> MGHHHHHHGENLYFQGSMHEHFDSIYLEFVDESYKPGKDEVIAVFRVTPAQGISIKDAAGRIAAESSVGTWTTLSVKPSWFEKLKAKAYRFHDLGDGSWLVWVAYPVELFEEGSIPNFASSILGNIFGMKAIAGLRVEDVYFPPSYLETFPGPNKGIQGVREILGIKDRPILATVPKPKLGYTPEEYGRVAYEILIGGIDLVKDDENFASQPFCRFEARLKEVMKAIDRAEKETGERKGYLANVTAPIREMEKRIKLVADYGNKFIMIDFLTAGWAALQHARELAEEYDLAIHGHRAFHAAFTRNPKHGVSMFLVAKLARMAGVDHVHVGTPGVGKMDAKTREVLEHTRIVREQYYRPKEGDLFHL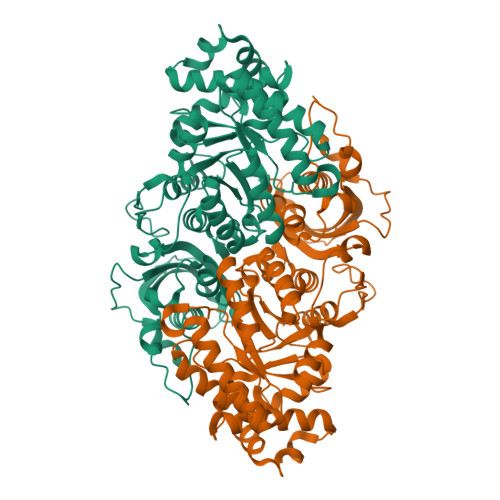EQPWSNIKPVFPVASGGLHPGTLPEVIRVMGKDIIMQVGGGVLGHPDGPEAGARAVRQAVEAAMKGISLDEYAREHRELARALEKWGYVRPV>MHHHHHHSSGRENLYFQGLQCIHIAEGHTKAVLCVDSTDDLLFTGSKDRTCKVWNLVTGQEIMSLGGHPNNVVSVKYCNYTSLVFTVSTSYIKVWDIRDSAKCIRTLTSSGQVTLGDACSASTSRTVAIPSGENQINQIALNPTGTFLYAASGNAVRMWDLKRFQSTGKLTGHLGPVMCLTVDQISSGQDLIITGSKDHYIKMFDVTEGALGTVSPTHNFEPPHYDGIEALTIQGDNLFSGSRDNGIKKWDLTQKDLLQQVPNAHKDWVCALGVVPDHPVLLSGCRGGILKVWNMDTFMPVGEMKGHD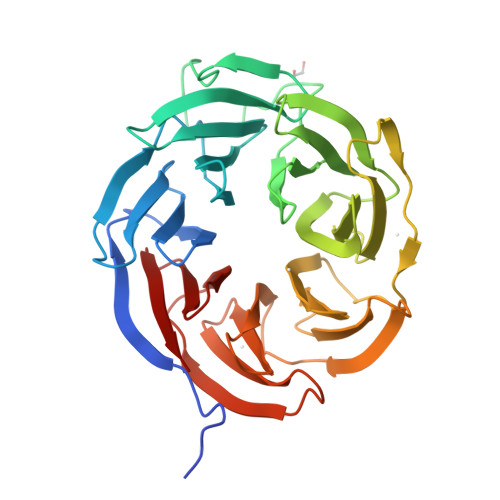SPINAICVNSTHIFTAADDRTVRIWKA[2x]> QVEAEVVTNGETSCSESTTQNDDGCRTRDDTRVSTNGSEDPEVAASGENKRANGNNSPSLSNGGFKPSRPPRPSRPPPPTPRRPASVNGSPSTNSDSDGSSTGSLPPTNTNVNTSTSEGATSGLIIPLTISGGSGPRPLNTVSQAPLPPGWEQRVDQHGRVYYVDHVEKRTTWDRPEPLPPGWERRVDNMGRIYYVDHFTRTTTWQRPTLESVRNYEQWQLQRSQLQGAMQQFNQRFIYGNQDLFATSQNKEFDPLGPLPPGWEKRTDSNGRVYFVNHNTRITQWEDPRSQGQLNEKPLPEGWEMRFTVDGIPYFVDHNRRATTYIDPRTGKSALDNGPQIAYVRDFKAKVQYFRFWCQQLAMPQHIKITVTRKTLFEDSFQQIMSFSPQDLRRRLWVIFPGEEGLDYGGVAREWFFLLSHEVLNPMYCLFEYAGKDNYCLQINPASYI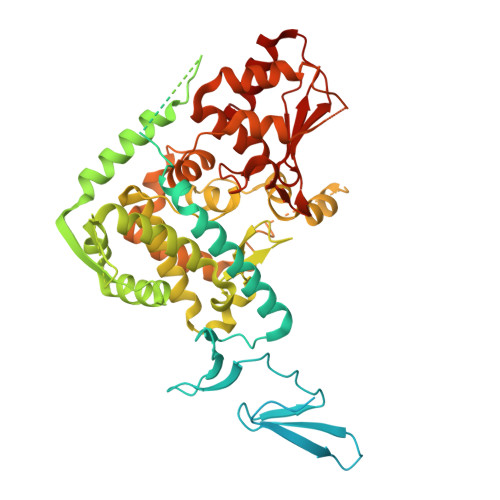NPDHLKYFRFIGRFIAMALFHGKFIDTGFSLPFYKRILNKPVGLKDLESIDPEFYNSLIWVKENNIEECGLEMYFSVDKEILGEIKSHDLKPNGGNILVTEENKEEYIRMVAEWRLSRGVEEQTQAFFEGFNEILPQQYLQYFDAKELEVLLCGMQEIDLNDWQRHAIYRHYTRTSKQIMWFWQFVKEIDNEKRMRLLQFVTGTCRLPVGGFADLMGSNGPQKFCIEKVGKENWLPRSHTCFNRLDLPPYKSYEQLKEKLLFAIEETEGFGQE> GTRVLIVGGSLVGLSTAVFLAHHDVPVTLVERHPGTSIHPRAVGYYPRTAELLATVGVEAPAKAAASGFEKHRTRAGVESLAGEVLFSKEELEGGDELADLTPSSLLLLPQDRLEPILRARAEELGAELRFGAELRSFTQDADGVSAVVRDADGGESVVRADYLVAADGPRSTVREALGIGREGRGVLSRHVSIAFGADFAAVLGERRYSVVHVQNDRVTGILVHDDTLTEGTLIVGYDPEKGEGLDDFTDARCAELVSAAIGSDDVAVTIRSRFPWDMAELVADAFVSDRVLVAGDAAHQIPPTGGYGANTGIADAFNLSWKLAHVLAGTAGRALLDTYDEERRPVGLYTARQGSLQLAVRSRTATEEQREAAHDAMRVTMGQAYPSGAFVADAGADPLPLTSDPRTLRGEPGTRAPYVVLERDGAPLSTLDLFGDGFVLLVGADGGSWAEAAGEAAAGLGVGIAFHRVAPDAGEGRPVDVHGRWAEAYGVGAAGAVLVRPDGIVAWRSRDGMPGGAGGRALTAALRTVLAR

Recently, two group A flavoprotein monooxygenases (FPMOs) (GrhO5 and GrhO6) and a flavoprotein oxidase (GrhO1) were shown to mediate the drastic remodeling of the 3 backbone and subsequent spiroketal pharmacophore formation. First, GrhO5 generates a ‐spiroketal moiety as part of the advanced intermediate dihydrolenticulone (4), which entails the rupture of three C−C bonds and a CO2 elimination step. The functional homolog RubL from rubromycin biosynthesis was shown to catalyze the same reaction sequence, pointing toward a universal strategy for spiroketal formation in the rubromycin family. In this work, the combined crystal structures of GrhO5 and RubL suggest three interconvertible catalytically relevant conformers, hereafter referred to as the “acceptor state” (FADox in OUT; accepts substrate, no reaction with NADPH), “reducible state” (FADox in OUT with bound substrate; reducible by NADPH) and the “catalytic state” (FADred in IN with bound substrate; reacts with O2 for hydroxylation).

To investigate the spiroketal synthases, the crystallization of GrhO5 and RubL was attempted under low‐salt conditions in the absence and presence of native substrate 3 and stable shunt product 7. While no RubL crystals formed under the tested conditions (however, crystals formed under high‐salt conditions, see below), yellow rod‐shaped crystals of native GrhO5 (without 3/7) were obtained after ca. 4–6 months that diffracted up to a resolution of 1.75 Å (for summary of all refinement statistics see Table S1) and enabled structural elucidation by molecular replacement. The GrhO5 structure obtained in the absence of substrate adopts the acceptor state (=resting state) similar to three closely related group A FPMOs from bacterial secondary metabolism (RdmE, anthracycline biosynthesis, RebC, rebeccamycin biosynthesis, PieE, piericidin A1 biosynthesis). Notably, the FAD‐OUT conformation in GrhO5 seems to be stabilized by a tryptophan residue (W281) that is properly positioned at the re‐side to engage in aromatic π‐π interactions with the isoalloxazine ring. The GrhO5‐type I enzymes including RdmE, PieE and RebC typically function as aromatic hydroxylases and exclusively feature this W fingerprint motif. Presumably, the observed CT complex is caused by the aromatic sandwich π‐π stacking of the indole ring of W281 (W289 in RubL) with FADox. Taken together, this provides strong evidence that the “OUT”‐conformation of the FAD observed in the crystal structure also predominates in solution. Hence, in the acceptor state of the spiroketal synthase without substrate, the direct reduction of FAD‐OUT and uncoupling are impeded. Hence, instead of being thermodynamically controlled, this kinetic effect may be caused by the gatekeeping W281/W289 side chain that sterically blocks the re‐side of FAD in the OUT conformation of RubL to prevent short‐range hydride transfer by NADPH in the acceptor state (as similarly proposed for RebC).> GKSTTLFSRHTKAIVWGMQTRAVQGMLDFDYVCSRDEPSVAAMVYPFTGDHKQKFYWGHKEILIPVFKNMADAMRKHPEVDVLINFASLRSAYDSTMETMNYAQIRTIAIIAEGIPEALTRKLIKKADQKGVTIIGPATVGGIKPGCFKIGNTGGMLDNILASKLYRPGSVAYVSRSGGMSNELNNIISRTTDGVYEGVAIGGDRYPGSTFMDHVLRYQDTPGVK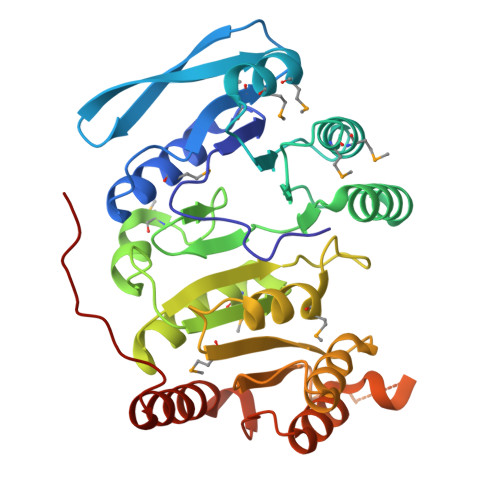MIVVLGEIGGTEEYKICRGIKEGRLTKPIVCWCIGTCATMFSSEVQFGHAGACANQASETAVAKNQALKEAGVFVPRSFDELGEIIQSVYEDLVANGVIVPAQEVPPPT> MEAPKMELKS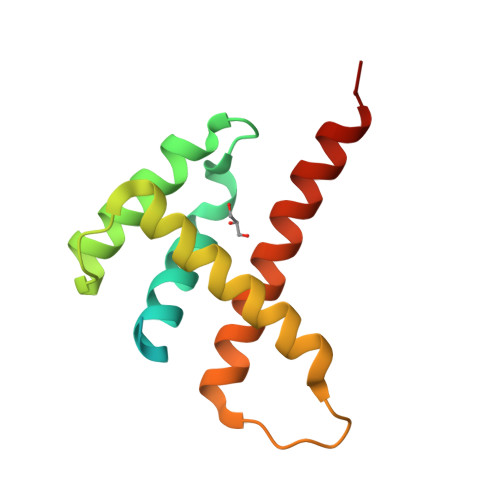YKRKNASLSPSSSPAKAQRTHLSLEEKIKLMRLVVRHKHELVDRKTSEFYAKIARIGYEDEGLAIHTESACRNQIISIMRVYEQRLAHRQPGMKTTPEEDELDQLCDEWKARLSELQQYREKFLVPR>MAIKIGINGFGRIGRLVLRVALGRKDIEVVAVNDPFIAPDYAAYMFKYDSTHGRYKGEVTASGDDLVIDGHKIKVFQERDPANIPWGKSGVDYVIESTGVFTKLEGAQKHIDAGAKKVIITAPSADAPMFVVGVNEDKYTPDLKIISNASCTTN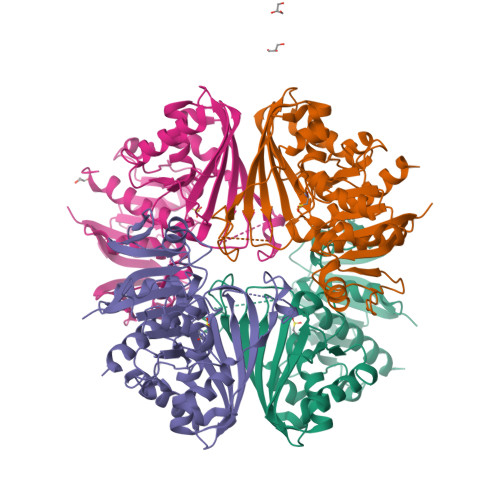CLAPLAKVVNDTFGIEEGLMTTVHSITATQKTVDGPSHKDWRGGRTASGNIIPSSTGAAKAVGKVIPELNGKLTGMSLRVPTTDVSVVDLTVRLKKAASYEEIAQAIKKASEGPLKGVLGYTEDAVVSTDFLGSSYSSIFDEKAGILLSPTFVKLISWYDNEYGYSTRVVDLLEHVAKASA[4x]>MKPARPCLVCSDEASGCHYGVLTCGSCKVFFKRAVEGQHNYLCAGRND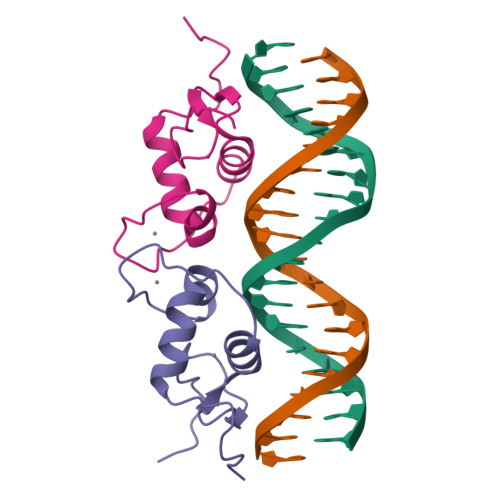CIIDKIRRKNCPACRYRKCLQAGMNLEARKTKK[2x]> TVGAVALDLDGNLAAATSTGGMTNKLPGRVGDSPLVGAGCYANNASVAVSCTGTGEVFIRALAAYDIAALMD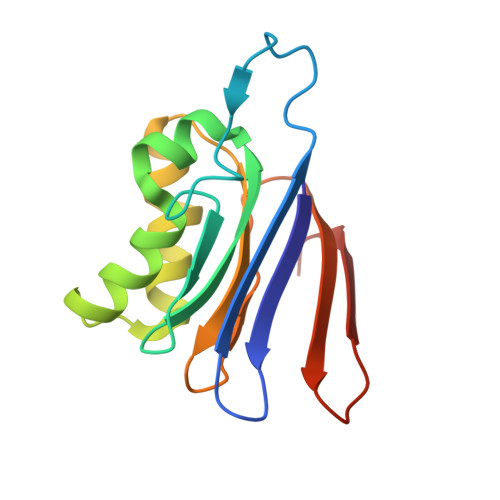YGGLSLAEACERVVMEKLPALGGSGGLIAIDHEGNVALPFNTEGMYRAWGYAGDTPTTGIYREKG>MHHHHHHTSVMSHEFQLATAETWPNPWPMYRALRDHDPVHHVVPPQRPEYDYYVLSRHADVWSAARDHQTFSSAQGLTVNYGELEMIGLHDTPPMVMQDPPVHTEFRKLVSRGFTPRQV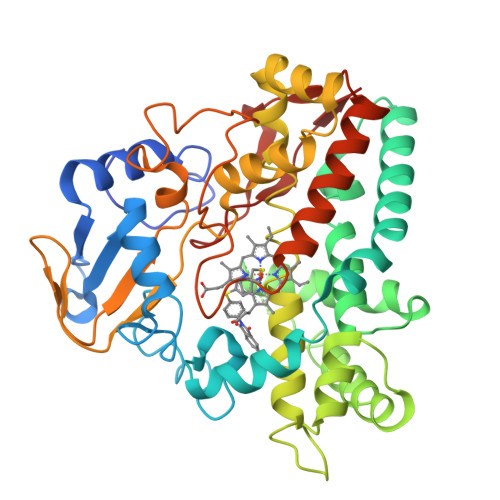ETVEPTVRKFVVERLEKLRANGGGDIVTELFKPLPSMVVAHYLGVPEEDWTQFDGWTQAIVAANAVDGATTGALDAVGSMMAYFTGLIERRRTEPADDAISHLVAAGVGADGDTAGTLSILAFTFTMVTGGNDTVTGMLGGSMPLLHRRPDQRRLLLDDPEGIPDAVEELLRLTSPVQGLARTTTRDVTIGDTTIPAGRRVLLLYGSANRDERQYGPDAAELDVTRCPRNILTFSHGAHHCLGAAAARMQCRVALTELLARCPDFEVAESRIVWSGGSYVRRPLSVPFRVTSSR[4x]>PEALERLAADPDREVRAAVAR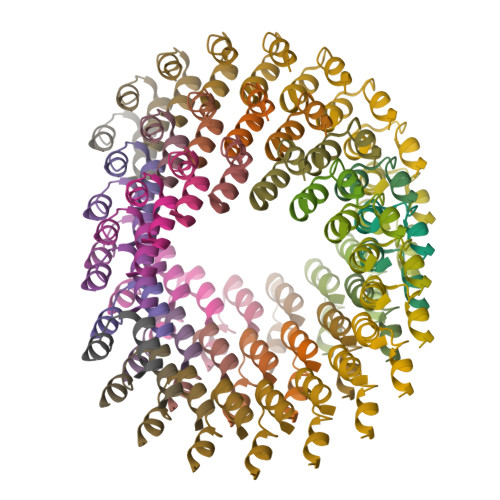RL[52x]> GPHMARKFFVGGNWKCNGTAEEVKKIVNTLNEAQV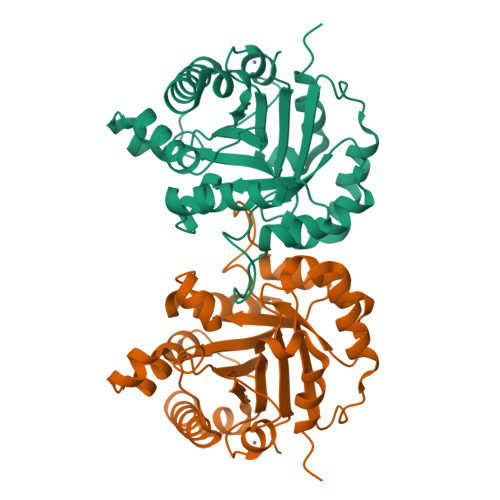PSQDVVEVVVSPPYVFLPLVKSTLRSDFFVAAQNCWVKKGGAFTGEVSAEMLVNLDIPWVILGHSERRAILNESSEFVGDKVAYALAQGLKVIACVGETLEEREAGSTMDVVAAQTKAIADRVTNWSNVVIAYEPVWAIGTGKVASPAQAQEVHDELRKWLAKNVSADVAATTRIIYGGSVNGGNDKELGGQADVDGFLVGGASLKPEFIDIIKAAEVKKSA> MSFVKDFKPQALGDTNLFKPIKIGNNELLHRAVIPPLTRMRALHPGNIPNRDWAVEYYTQRAQRPGTMIITEGAFISPQAGGYDNAPGVWSEEQMVEWTKIFNAIHEKKSFVWVQLVVLGWAAFPDNLARDGLRYDSASDNVFMDAEQEAKAKKANNPQHSLTKDEIKQYIKEYVQAAKNSIAAGADGVEIHSANGYLLNQFLDPHSNTRTDEYGGSIENRARFTLEVVDALVEAIGHEKVGLRLSPYGVFNSMSGGAETGIVAQYAYVAGELEKRAKAGKRLAFVHLVEPRVTNPFLTEGEGEYEGGSNDFVYSIWKGPVIRAGNFALHPEVVREEVKDKRTLIGYGRFFISNPDLVDRLEKGLPLNKYDRDTFYQMSAHGYIDYPTYEEA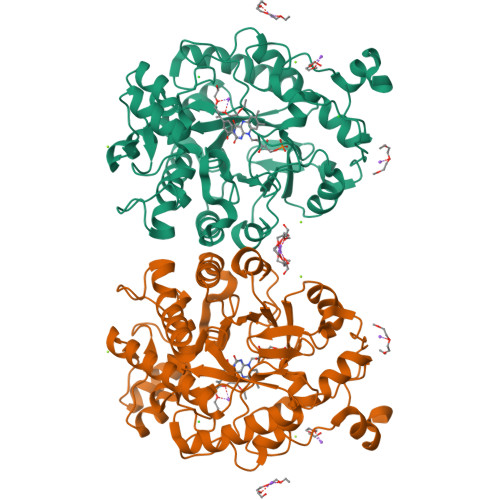LKLGWDKK>[2x]GAMNPDPEATMDRSLLQRQDLPYRFSAVDLDSVDGQRHYRLWLGRPLQAPPAAGYPVVWMLDGNAAVGALDESTLRRLADGDAPLLVAIGYRTPLRIDRAGRTFDYTPASPGQADQRDPLNGLPSGGADAFLDLLRDGMRPAVAAQ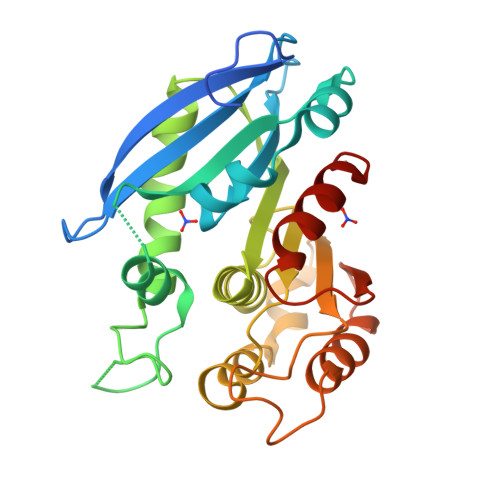APLDTARQTLWGHSYGGLLVLHALFTRPGEFARYAAASPSLWWRDGAILGERAGLEQRLRGKRAELLLWRGSAEPASPRGSLKAEPGQAMARLVDDLRRVAGLTLDFQPLDGLGHGETLGASLRLLLARPAVERQR> MSNYVIQADQQLLDALRAHYEGALSDRLPAGALFAVKRPDVVITAYRSGKVLFAGKAAEQEAAKWISGASASNETADHQPSALAAHQ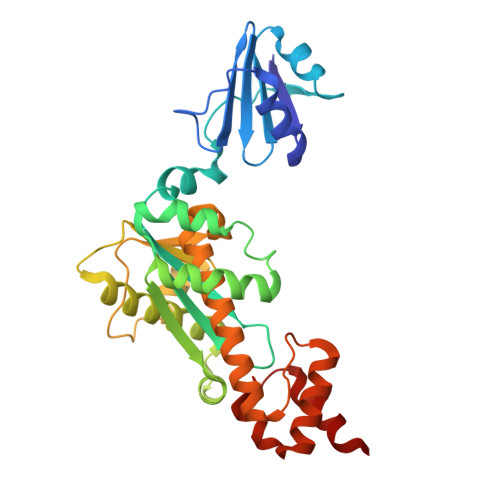LGSLSAIGSDEVGTGDYFGPIVVAAAYVDRPHIAKIAALGVKDSKQLNDEAIKRIAPAIMETVPHAVTVLDNPQYNRWQRSGMPQTKMKALLHNRTLVKLVDAIAPAEPEAIIIDEFLKRDSYFRYLSDEDRIIRERVHCLPKAESVHVSVAAASIIARYVFLEEMEQLSRAVGLLLPKGAGAIVDEAAARIIRARGEEMLETCAKLHFANTKKALAIAKRRK> PAKKPYNKIVSHLLVAEPEKIYAMPDPTVPDSDIKALTTLCDLADRELVVIIGWAKHIPGFSTLSLADQMSLLQSAWMEILILGVVYRSLSFEDELVYADDY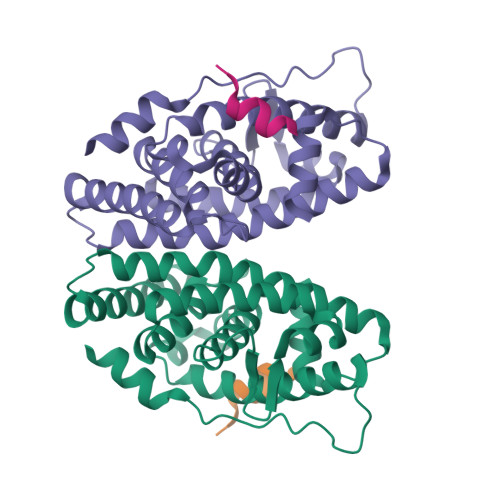IMDEDQSKLAGLLDLNNAILQLVKKYKSMKLEKEEFVTLKAIALANSDSMHIEDVEAVQKLQDVLHEALQDYEAGQHMEDPRRAGKMLMTLPLLRQTSTKAVQHFYNIKLEGKVPMHKLFLEMLEAKV;> LERNNIKQAANNSLLLHLLKSQTIP Salmonella enterica serovar Typhimurium (S. Typhimurium), a gram-negative bacterium responsible for innumerable cases of acute gastroenteritis worldwide, utilizes two T3SSs, encoded within its pathogenicity islands 1 (SPI-1) and 2 (SPI-2), to invade cells and establish an intracellular replicative niche. The core component of this machine is the envelope-associated needle complex, which consists of a multiring base, an inner rod, and a needle filament extension that protrudes several nanometers from the bacterial surface. The entire structure is traversed by an approximately 2-nm channel that serves as a conduit for the T3SS protein substrates as they pass through the bacterial envelope. Furthermore, four residues at the end of the C-terminal α-helix, three charged (K66, D70, and R80) and one polar uncharged (Q77), form the lumen of the channel and create an electrostatic surface potential of alternating charges, which spiral upwardly about the needle, a feature that has been proposed to be important for substrate translocation.

As it is possible that constrains imposed on the filaments by their tight association to the base could result in structural differences, we sought to obtain structural information for needle filaments attached to the base substructure. Fully assembled needle complexes isolated by affinity chromatography were subjected to cryo-EM analysis. PrgI needles were boxed out from fully assembled, intact needle complexes and segmented into square particles for 2D classification. The α-helices in each PrgI subunit and their N-terminal loops pointing to the solvent were clearly resolved in 2D class averages of the helical filaments. The helical parameters, rise and twist, determined by helical indexing of the averaged power spectrum were measured to be 4.24 Å and 63.35°, respectively, which are in close agreement with the previously reported values for the cryo-EM structure of isolated needle filaments. By applying helical symmetry in the EM reconstruction, we obtained a 3D map of the needle filament at 3.7 Å resolution as determined by the Fourier shell correlation (FSC) at 0.143 cutoff. The first two residues of PrgI are flexible and could not be resolved in our map, although the 3D map allowed the unambiguous building of most of the side chains. The resulting atomic model is in good agreement with the cryo-EM structure of isolated needle filaments, except for a slightly smaller rise (4.24 Å versus 4.33 Å in isolated needle filaments) in the helical parameters. The structure of the PrgI monomer extracted from the cryo-EM structure of filaments attached to the base is also entirely consistent with the structure of the monomer extracted from the cryo-EM structure of isolated needle filaments (the Cα root mean square deviation [RMSD] is 0.509 Å over 78 residues).

>[19x]MATPWSGYLDDVSAKFDTGVDNLQTQVTEALDKLAAKPSDPALLAAYQSKLSEYNLYRNAQSNTVKVFKDIDAAIIQNFR Multi-subunit SMC complexes control chromosome superstructure and promote chromosome disjunction, conceivably by actively translocating along DNA double helices. SMC subunits comprise an ABC ATPase “head” and a “hinge” dimerization domain connected by a 49 nm coiled-coil “arm. The heads undergo ATP-dependent engagement and disengagement to drive SMC action on the chromosome. Here, we elucidate the architecture of prokaryotic Smc dimers by high-throughput cysteine cross-linking and crystallography.

A structure of a Smc middle segment, designated as BsSmcCC2, comprising residues 246–379 and 793–929 connected via a short linker, was solved by crystallography at a resolution of 3.2 Å. The BsSmcCC2 monomer comprises two ∼120 residues long α helices (designated as αN1 and αC1), whose arrangement presents the knob-into-hole organization of a canonical coiled coil. The asymmetric unit is formed by two dimers of BsSmcCC2. In each dimer, the two molecules are aligned side by side along a pseudo-symmetry axis, which is reminiscent of the hinge-proximal Smc rod structure (Soh et al., 2015). In the middle of BsSmcCC2, residues of αN1 located in heptad positions “b,” “e,” and “f” are involved in the contact between the two coiled coils via charged and hydrophobic side chains. At the top of the structure, residues of αC1 form a similar dimer interface. To establish whether the organization of the BsSmcCC2 dimer in the crystal is compatible with the cysteine cross-linking pattern described above, we mapped the cross-linking efficiency onto the BsSmcCC2 structure and plotted it against the corresponding Cα-Cα distances (respectively). The excellent agreement between the crystal structure and the in vivo cross-linking pattern implies that both datasets faithfully represent the architecture of Smc-ScpAB complexes in vivo.

>[4x]GSGMEKVQMAKEEELAESSAISAKEAKIEDTRDKIQALDESVDELQQVLLVTSEELEKLEGRKEVLKERKKNAVQNQEQLEEAIVQFQQKETVLKEELSKQEAVFETLQAEVKQLRAQVKEKQQALSLHNENVEEKIESGGSGGSRLTKQKQTQSSTKESLSNELTELKIAAAKKEQACKGEEDNLARLKKELTETELALKEAKEDLSFLTSEMSSSTSGEEKLEEAAKHKLNDKTKTIELIALRRDQRIKLQHGLDTYERELKEMKRLYKQKTTLLKDEEV> MHHHHHHENLYFQGTKDLNTLVSELPEIYQTIFGHPEWDGDAARDCNQRLDLITEQYDNLSRALGRPLNVLDLGCAQGFFSLSLASKGATIVGIDFQQENINVCRALAEENPDFAAEFRVGRIEEVIAALEEGEFDLAIGLSVFHHIVHLHGIDEVKRLLSRLADVTQAVI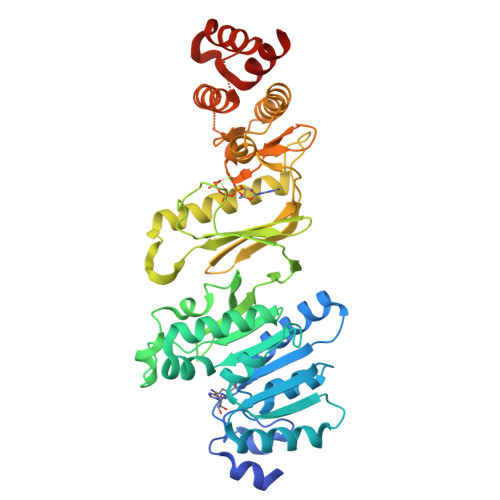LELAVKEEPFYWGVSQPDDPRELIEQCAFYRLIGEFDTHLSPVPRPMYLVSNHRVLINDFNQPFQHWQNQPYAGAGLAHKRSRRYFFGEDYVCKFFYYDMPHGILTAEESQRNKHELHNEIKFLTQPPAGFDAPAVLAHGENAQSGWLVMEKLPGRLLSDMLAAGEEIDREKILGSLLRSLAALEKKGFWHDDVRPWNVMVDARQHARLIDFGSIVTTPQDCSWPTNLVQSFFVFVNELFAENKSWNGFWRSAPVHPFNLPQPWSNWLYAVWQEPVERWNFALLLALFEKKAKLPSAEQQ>[5x]AELPPGRLATTEDYFAQQAKQAVTPDVMAQLAYMNYIDFISPFYSRGCSFEAWELKHTPQRVIKYSIAFYAYGLASVALIDPKLRALAGHDLDIAVSKMKCKRVWGDWEEDGFGTDPIEKENIMYKGHLNLMYGLYQLVTGSRRYEAEHAHLTRIIHDEIAANPFAGIVCEPDNY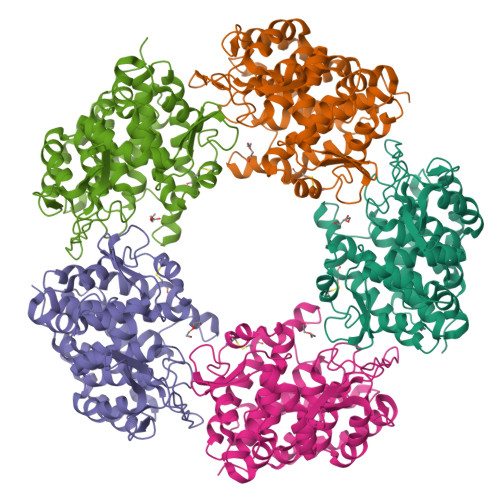FVQCNSVAYLSLWVYDRLHGTDYRAATRAWLDFIQKDLIDPERGAFYLSYHPESGAVKPWISAYTTAWTLAMVHGMDPAFSERYYPRFKQTFVEVYDEGRKARVRETAGTDDADGGVGLASAFTLLLAREMGDQQLFDQLLNHLEPPAKPSIVSASLRYEHPGSLLFDELLFLAKVHAGFGALLRMPPPAAKLAGK>[3x]GAMAMSDLPIEFTELVDLMSLGISPQFLDFRSTTFESDHFVTVRETKDGTNSVAIVDLAKGNEVTRKNMGGDSAIMHPSQMVISVRANGTIVQIFNLETKSKLKSFTLDEPVIFWRWLSETTLGFVTARSILTSNVFDGNVNAKPQLLTLRHANLNNTQIINFVANKNLDWFAVVGILQENGRI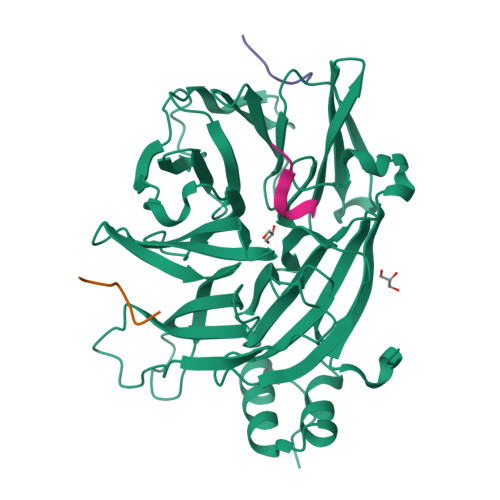AGRIQLFSKQRNISQAIDGHVAIFTNILLEGNGSTPVQVFVTGNRNATTGAGELRIIEIDHDASLPSQYQKETTDIFFPPDATNDFPIAVQVSEKYGIIYLLTKYGFIHLYELETGTNLFVNRITAESVFTAAPYNHENGIACINKKGQVLAVEISTSQIVPYILNKLSNVALALIVATRGGLPGADDL;>[9x]GVSLIDL> MGTNPPSPQDVEEILDQGVEEVDRIVSGLGELH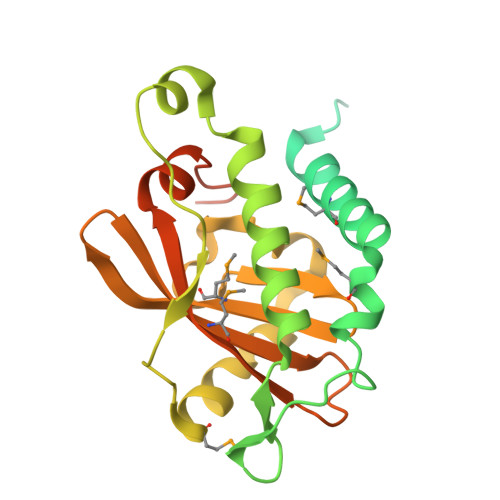GAGDHPGQQQDVAESVARERPESSQGGGVAKRPRISHDTPGSSGARSPDYSVETDIPYHTELLSDMERVIEDNEMAHIFSASSSTGEVLYSPSVFHATEKQKNAALSLLEERYKRDFPHDLAENIVIRDIEFVDGNIPSMLDIFTRRSVLKLLGYSAWDEGLGKQIFFDVGEYRVNMFPLRIEEGFHLRQMVAYHLQEANPRYLWLGTVRIQSVLIENIGYATNPARHSTQSADRAGPGPHHHHHH(2~{R})-2-[(1-azanylisoquinolin-6-yl)amino]-2-(5-ethoxy-2-fluoranyl-phenyl)-1-[(2~{R})-2-phenylpyrrolidin-1-yl]ethanone | C29 H29 F N4 O2 | 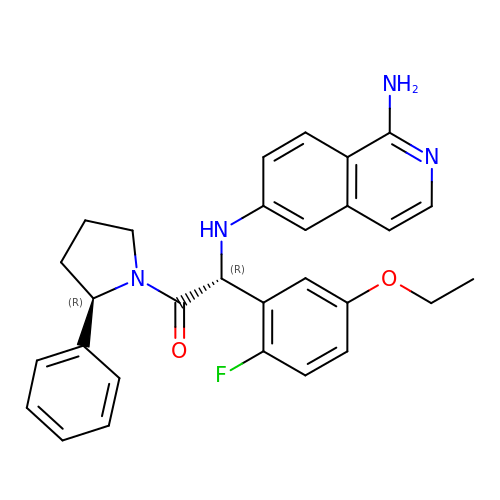KYHMCMPFXIGNJI-KAYWLYCHSA-N> GIEASLLTDPKDVSGRTVDYIIAGGGLVGLTTAAKLTENPNISVLVIESGSYESDRGPIIEDLNAYGDIFGSSVDHAYETVELATNNQTALVRSGNGLGGSTLINGGTWTRPHKAQVDSWETVFGNEGWNWDNVAAYSLQAERARAPNAKQIAAGHYFNTSCHGVNGTVHAGPRDTGDDYSPIVKALMSAVEDRGVPTKKDFGCGDPHGVSMFPNTLHEDQVRSDAAREWLLPNYQRPNLQVLTGQYVGKVLLSQNGTTPRAVGVEFGTHKGNTHNVYAKHEVLLAAGSAVSPTILEYSGIGMKSILEPLGIDTVVDLPVGLNLQDQTTATVRSRITSAGAGQGQAAWFATFNETFGDYSEKAHELLNTKLEQWAEEAVARGGFHNTTALLIQYENYRDWIVNHNVAYSELFLDTAGVASFDVWDLLPFTRGYVHILDKDPYLHHFAYDPQYFLNELDLLGQAAATQLARNISNSGAMQTYFAGETIPGDNLAYDADLSAWTEYIPYHFRPNYHGVGTCSMMPKEMGGV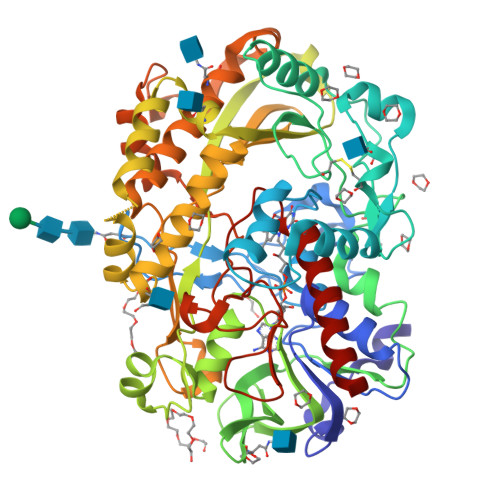VDNAARVYGVQGLRVIDGSIPPTQVSSHVMTVFYAMALKISDAILEDYASMQ The ZUFSP family, with ZUP1 as its sole human member, has a modular architecture with a core catalytic domain highly active against the ubiquitin-derived peptide RLRGG, but not against ubiquitin itself. A hallmark of ZUFSP proteins is a papain-fold catalytic core domain with the catalytic Cys–His–Asp triad and two conserved acidic residues recognizing the two C-terminal arginine residues of ubiquitin within the RLRGG motif. Except for the minimalistic Mug105 from S. pombe, all ZUFSP family members contain a number of N-terminal ubiquitin-binding domains, which are dispensable for catalysis itself, but are required for chain cleavage. Biochemical and structural studies suggest that the acquisition of two family-specific proximal domains have changed the default K48 preference of the ZUFSP family to the K63 preference observed in ZUP1 and its insect homolog.

Like mammals, the fission yeast Schizosaccharomyces pombe encodes a single ZUFSP family member, Mug105, which is much shorter than human ZUP1 and lacks all recognizable ubiquitin-binding domains. Interestingly, this fungal protein preferentially cleaves K48-linked ubiquitin chains. Since sequence analysis of Mug105 did not identify any ubiquitin-binding domains, we set out to investigate the basis of Mug105 specificity by solving the crystal structure of full-length Mug105 to a resolution of 2.0 Å. The asymmetric unit contained two Mug105 molecules. Mug105 assumes a globular α/β papain-fold structure. The active site residues (Cys-42, His-165, and Asp-183) assume a geometry similar to other papain-fold cysteine proteases. Overall, the Mug105 structure bears a striking resemblance to the ZUP1 catalytic core domain, with an RMSD of 1.7 Å over 215 residues. As predicted by sequence analysis, all ubiquitin-binding domains of ZUP1 are absent from Mug105, and no additional UBD candidates are apparent from the structure. The Mug105 structure does not contain ubiquitin, but the recognition site of the ubiquitin C-terminal R-x-R motif appears to be conserved between ZUP1 and Mug105. The corresponding Trp-104 of the ubiquitin-less Mug105 structure is mainly adopting a conformation blocking the substrate-binding cleft.

>[2x]MSKCLQQLKRQLQHFGIDGCSLADGDIDYFFTVTGIDRGWGCGWRNIQMLISWLQYTNPNWFKRNFSSGNYEINSLQSLLLSAWMKGIDAEGYAQLGDNLHGKWIGATEVYSLFTGLFVNVALVDFDFRSEASASNALFLYVKKHFESSNDTSNVSPCYLQFQGHSIIIIGFCSSLETLVVLDPDRYQSVQKKFVNIADFNHCYMRKKRSLKFSQFQLVHFKQNIFLNDFSSKLEVRSTRISDF>GDICIKDSINTLWTGIKPPPNCQIVENTDTNDGKLTLVLV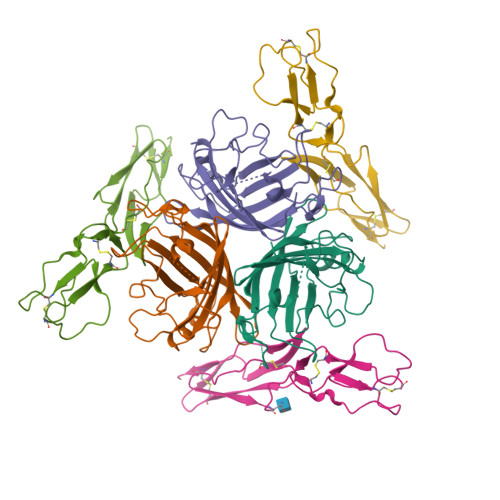KNGGLVNGYVSLVGVSDTVNQMFTQKSATIQLRLYFDSSGNLLTDESNLKIPLKNKSSTATSEAATSSKAFMPSTTAYPFNTTTRDSENYIHGICYYMTSYDRSLVPLNISIMLNSRTISSNVAYAIQFEWNLNAKESPESNIATLTTSPFFFSYIREDDN[12x];>CEEPPTFEAMELIGKPKPYYEIGERVDYKCKKGYFYIPPLATHTICDRNHTWLPVSDDACYRETCPYIRDPLNGQAVPANGTYEFGYQMHFICNEGYYLIGEEILYCELKGSVAIWSGKPPICEKV[12x]>MHHHHHHMFSRFSNVVSEIEKKYVDKISISEIMTKAIEGLLSNLDAHSAYLNEKKFKEFQAQTEGEFGGLGITVGMRDGVLTVIAPLEGTPAYKAGVKSGDNILKINNESTLSMSIDDAINLMRGKPKTPIQITIVRKNEPKPLVFNIIRDIIKLPSVYVKKIKETPYLYVRVSGFDKNVTKSVLEGLKANPKAKGIVLDLRGNPGGLLNQAVGLSNLFIKEGVLVSQKGKNKEESLEYKANGRAPYTNLPIAVLVNGGSASASEIVAGALQDHKRAVIIGEKTFGKGSVQMLLPVNKDEAIKITTARYYLPSGRTIQAKGITPDIVIYPGKVPEN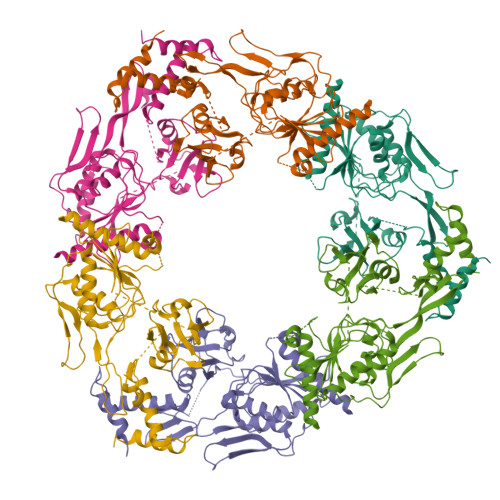ENKFSLKEADLKHHLEQELKKLDDKTPNSKEADKDKKNEEEKEVTPKMINDDIQLKTAIDSLKTWSIVDEKMDEKAPKKK[6x]>MRRTKEDSEKTRTAILLAAEELFLEKGVSHTSLEQIARAAGVTRGAVYWHFQNKA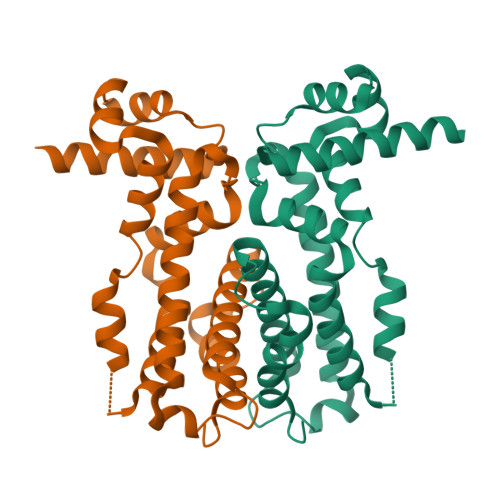HLFNEMLNQVRLPPEQLTERLSGCDGSDPLRSLYDLCLEAVQSLLTQEKKRRILTILMQRCEFTEELREAQERNNAFVQMFIELCEQLFARDECRVRLHPGMTPRIASRALHALILGLFNDWLRDPRLFDPDTDAEHLLEPMFRGLVRDWGQASSAP[8x]>[7x]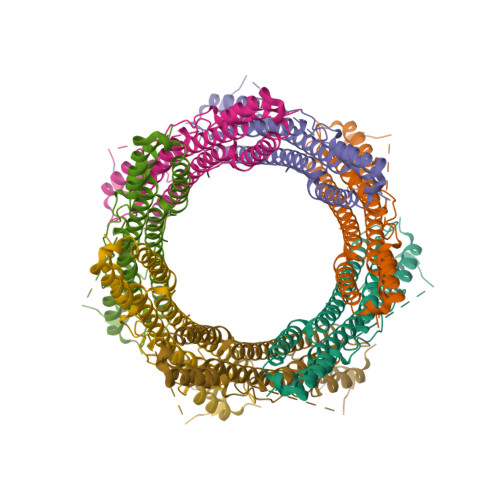MTQSQTVTVDQQEILNRANEVEAPMADPPTDVPITPCELTAAKNAAQQLVLSADNMREYLAAGAKERQRLATSLRNAAKAYGEVDEEAATALDNDGEGTVQAESAGAVGGDSSAELTDTPRVATAGEPNFMDLKEAARKLETGDQGASLAHFADGWNTFNLTLQGDVKRFRGFDNWEGDAATACEASLDQQRQWILHMAKLSAAMAKQAQYVAQLHVWARREHPTYEDIVGLERLYAENPSARDQILPVYAEYQQRSEKVLTEYNNKAALEPVNPPKPPPAIKIDPPPPPQEQGLIPGFLMPPSDGSGVTPGTGMPAAPMVPPTGSPGGGLPADTAAQLTSAGREAAALSGDVAVKAASLGGGGGGGVPSAPLGSAIGGAESVRPAGAGDIAGLGQGRAGGGAALGGGGMGMPMGAAHQGQGGAKSKGSQQEDEALYTEDRAWTEAVIGNRRRQDSKESK methyl 4-{3-[(5-methyl-1,2-oxazole-3-carbonyl)amino]phenyl}butanoate | C16 H18 N2 O4 | 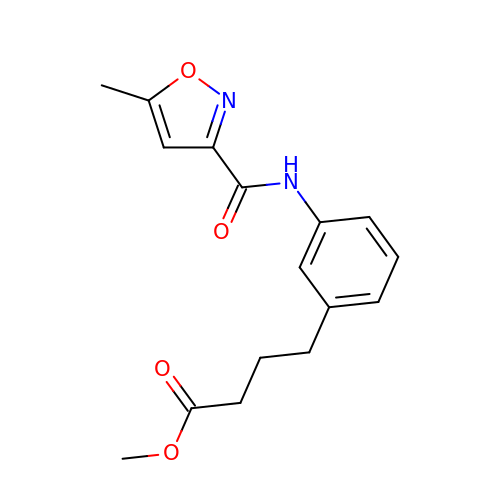QXRDFNLRULOJRX-UHFFFAOYSA-N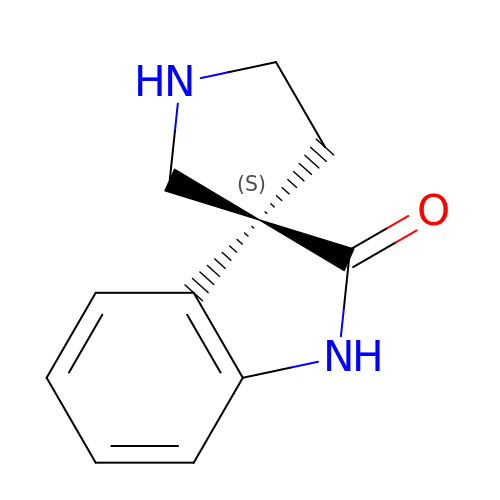(3S)-spiro[indole-3,3'-pyrrolidin]-2(1H)-one | C11 H12 N2 O | FQSHLSLQUHZOMV-LLVKDONJSA-N>GSMTIKLLDEFLKKHDLTRYQLSKLTGISQNTLKDQNEKPLNKYTVSILRSLSMISGLSVSDVLFELEDIEKNSDDLAGFKHLLDKYKLSFPAQEFELYCLIKEFESANIEVLPFTFNRFENEEHVNIKKDVCKALENAITVLK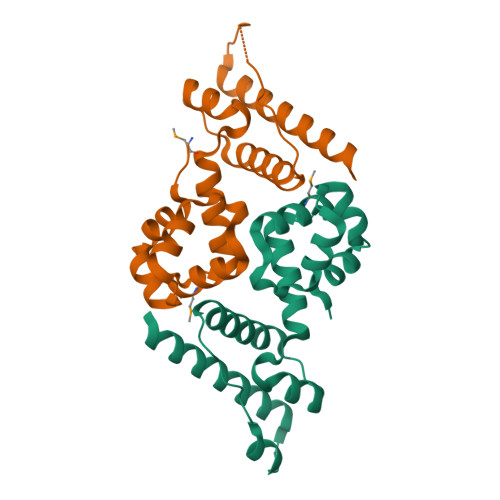EKKNELL[2x]> NGIVPDAGHQGPDVSAVNGGTQVINIVTPNNEGISHNQYQDFNVGKPGAVFNNALEAGQSQLAGHLNANSNLNGQAASLILNEVVSRNPSFLLGQQEVFGIAAEFVLSNPNGITCDGCGFINTSRSSLVVGNPLFENG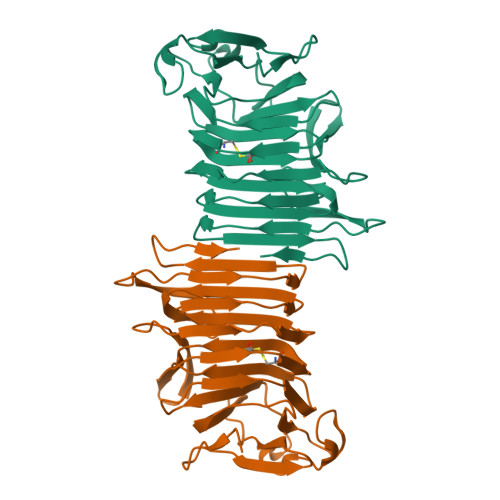QLKGYSTLNNTNLLSLGKNGLNTTGLLDLIAPRIDSRGKITAAEISAFTGQNTFSQHFDILSSQKPVSALDSYFFGSMQSGRIRIINTAEGSGVKLAGHHHHHH> GGSAQE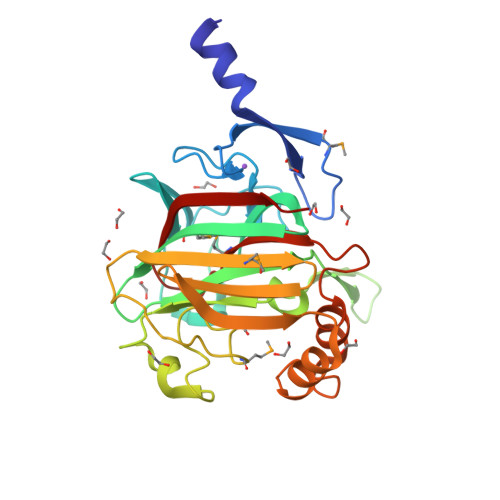EQSANEVAVSYSKSLKAAEMDSLQLPVDADGYITIFDGKTFNGWRGYGKDRVPSKWTIEDGCIKFNGSGGGEAQDGDGGDLIFAHKFKNFELEMEWKVSKGGNSGIFYLAQEVTSKDKDGNDVLEPIYISAPEYQVLDNDNHPDAKLGKDNNRQSASLYDMIPAVPQNAKPFGEWNKAKIMVYKGTVVHGQNDENVLEYHLWTKQWTDLLQASKFSQDKWPLAFELLNNCGGENHEGFIGMQDHGDDVWFRNIRVKVLD>[2x]ADNLAEFHVQNQECDSCHTPDGELSNDSLTYENTQCVSCHGTLAEVAETTKHEHYNAHASHFPGEVACTSCHSAHEKSMVYCDSCHSFDFNMPYAKKWLRDEPTIAELAKDKSERQAALASAPHDTVDVVVVGSGGAGFSAAISATDSGAKVILIEKEPVIGGNAKLAAGGMNAAWTDQQKAKKITDSPELMFEDTMKGGQNINDPALVKVLSSHSKDSVDWMTAMGADLTDVGMMGGASVNRAHRPTGGAGVGAHVVQVLYDNAVKRNIDLRMNTRGIEVLKDDKGTVKGILVKGMYKGYYWVKADAVILATGGFAKNNERVAKLDPSLKGFISTNQPGAVGDGLDVAENAGGALKDMQYIQAHPTLSVKGGVMVTEAVRGNGA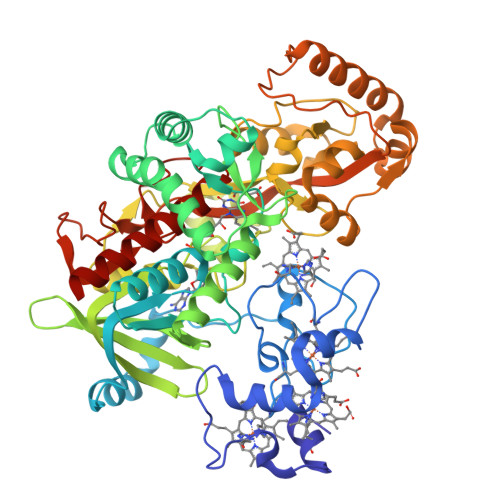ILVNREGKRFVNEITTRDKASAAILAQTGKSAYLIFDDSVRKSLSKIDKYIGLGVAPTADSLVKLGKMEGIDGKALTETVARYNSLVSSGKDTDFERPNLPRALNEGNYYAIEVTPGVHYTMGGVMIDTKAEVMNAKKQVIPGLYGAGEVTGGVHGANRLGGNAISDIITFGRLAGEEAAKYSKKN> SMS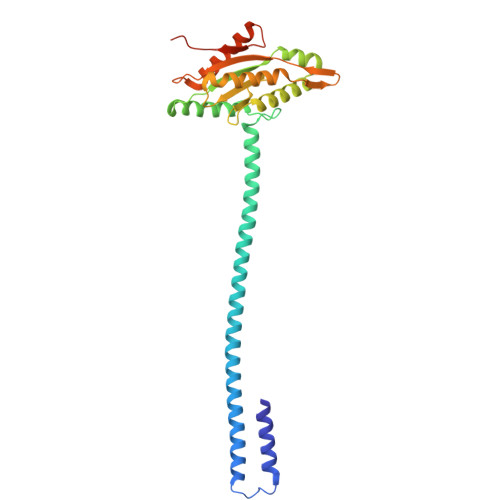RERELDAWIDGLLADPQFHGHPLHQALARLRQQSLEQLVRLERIARISDGFQSMAREQNLSLSERYHKQLRRLEKVARISDRYQQMMRDLNLALKEASIRDPLTGLPNRRMLLERLREENERSQRHGQSYVLAMLDVDFFKQVNDTWGHDSGDRVLVEIARAMESELREYDLCGRWGGEEFLLLLPQTRLQDAGPVLERVRDSVRTLAVRVGTEALSVTASVGVTEHRIGETYSQTVNRADAALLDAKRSGRDKCVFAALPPLPAPSRPAPAR> MLKEWMIFTCSLLTLAGASLPLSGCISRGQESISEGAAFGAGILREPGATKKADTKDLNVPPPVYGPPQVIFRIDDNRYFTLENYTHCENGQTFYNNKAKNIHVKILDASGYLFKGRLFWLSTRDDFLAFPATLNTRHASCMGSNKGCMNAVIVTTDGGKRRSGVPYGSYTQNPTGATRDYDMLVMNDGF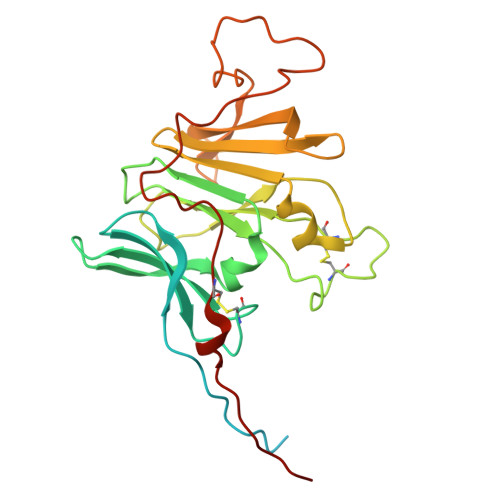YLLRYRGGQGRFSPVILRWILSTEDSSGVVRSEDAYELFRPGEEVPSTGFYKIDLSRFYPKNNVMEMQCDRTLEPVQPSESKIQ>[2x]GSHELLSKEEEEAKAKADKIKLALEKLKEAKVKKLVVKVHMDDSSTKSLMVDERQLARDVLDNLFEKTHCDC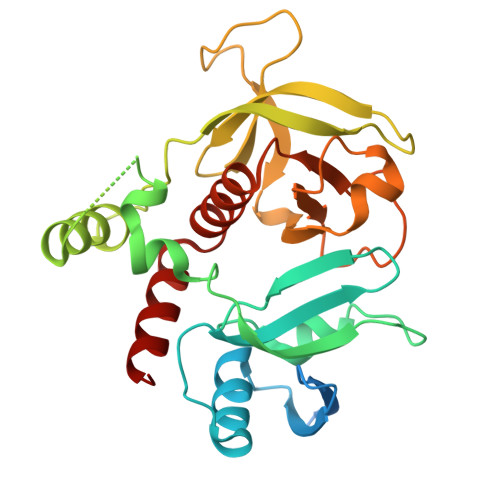NVDWCLYEIYPELQIERVFEDHENVVEVLSDWTRDTENKVLFLEKEERYAVFKNPQNFYLDNKGKKENKETNEKMNAKNKEYLLEESFCGTSIIVPELEGALYLKEDGKKSWKRRYFLLRASGIYYVPKGKTKTSRDLACFIQFENVNIYYGIQCKMKYKAPTDHCFVLKHPQIQKESQYIKYLCCDDARTLSQWVMGIRIAKYGKTLYDNYQRAVARA> MFKKLINKKNTINNYNEELDSSNIPEHIAIIMDGNGRWAKKRKMPRIKGHYEGMQTIKKITRIASDIGVKYLTLYAFSTENWSRPESEVNYIMNLPVNFLKTFLPELIEKNVKVETIGFTDKLPKSTIEAINNAKEKTANNTGLKLIFAINYGGRAELVHSIKNMFDELHQQGLNSDIIDETYINNHLMTKDYPDPELLIRTSGEQRISNFLIWQVSYSEFIFNQKLWPDFDEDEL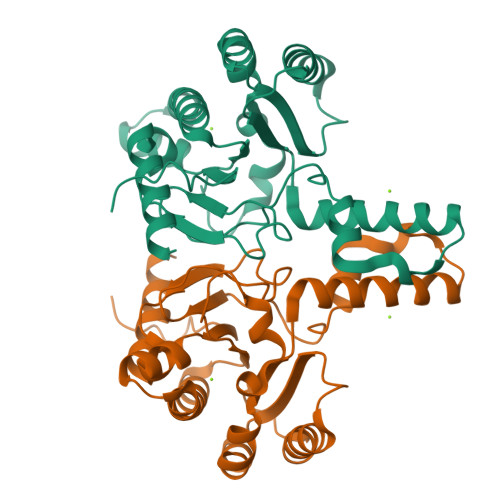IKCIKIYQSRQRRFGGLSEE> MERTELLKPRTLADLIRILHELFAGDEVNVEEVQAVLEAYESNPAEWALYAKFDQYRYTRNLV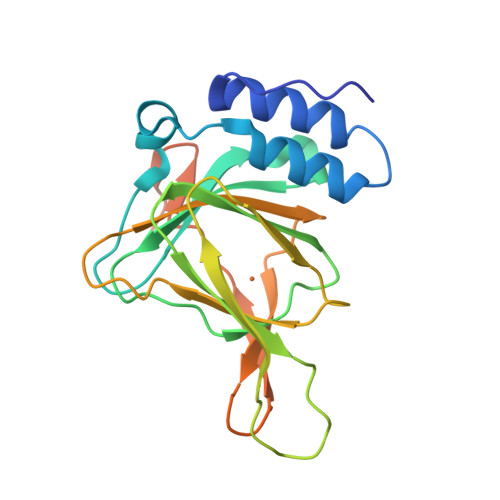DQGNGKFNLMILCWGEGHGSSIHDHTDSHCFLKLLQGNLKETLFDWPDKKSNEMIKKSERTLRENQCAYINDSIGLHRVENVSHTEPAVSLNLYSPPFDTCHAFDQRTGHKNKVTMTFHSKFGIRTPFTTSGSLENNSAWSHPQFEK>MALVDGFLELERSSGKLEWSAILQKMASDLGFSKILFGLLPKDSQDYENAFIVGNYPAAWREHYDRAGYARVDPTVSHCTQSVLPIFWEPSIYQTRKQHEFFEEASAAGLVYGLTMPLHGARGELGALSLSVEAENRAEANRFMESVLPTLWMLKDYALQSGAGLA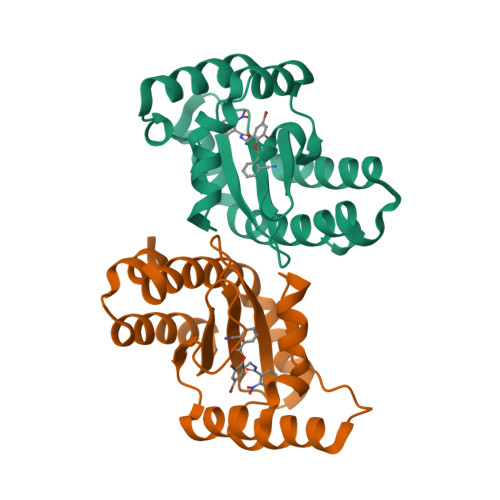FEH[2x]>SNAMRILIISDVHANLVALEAVLSDAGRVDDIWSLGDIVGYGPRPRECVELVRVLAPNISVIGNHDWACIGRLSLDEFNPVARFASYWTTMQLQAEHLQYLESLPNRMIDGDWTVVHGSPRHPIWEYIYNARIAALNFPAFDTPLCFVGHTHVPLYIREDEALSNVAPHHPNDGEVLDVSSGRYIINPGAVGQPRDGDPRASY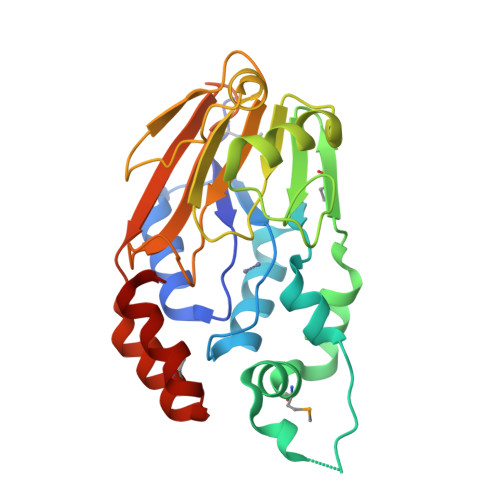AIFEPDAQRVTFHRVEYRIADTQAQMREAGLPESLVTRLAAGV[3x]> MTMATTAMNVSVPPPDEEEQLLAKFVFGDTTD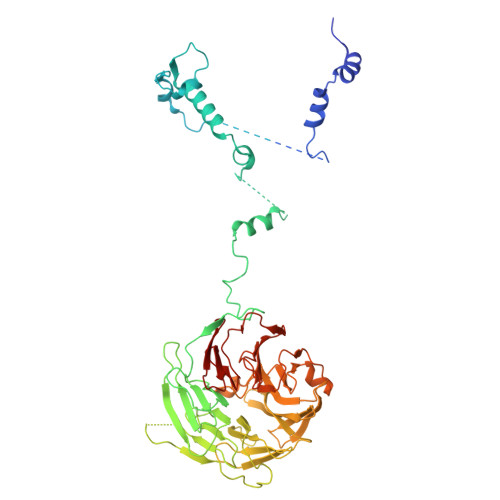LQENLAKFNADFIFNEQEMDVEDQEDEGSESDNSEEDEAQNGELDHVNNDQLFFVDDGGNEDSQDKNEDTMDVDDEDDSSSDDYSEDSEEAAWIDSDDEKIKVPILVTNKTKKLRTSYNESKINGVHYINRLRSQFEKIYPRPKWVDDESDSELDDEEDDEEEGSNNVINGDINALTKILSTTYNYKDTLSNSKLLPPKKLDIVRLKDANASHPSHSAIQSLSFHPSKPLLLTGGYDKTLRIYHIDGKTNHLVTSLHLVGSPIQTCTFYTSLSNQNQQNIFTAGRRRYMHSWDLSLENLTHSQTAKIEKFSRLYGHESTQRSFENFKVAHLQNSQTNSVHGIVLLQGNNGWINILHSTSGLWLMGCKIEGVITDFCIDYQPISRGKFRTILIAVNAYGEVWEFDLNKNGHVIRRWKDQGGVGITKIQVGGGTTTTCPALQISKIKQNRWLAVGSESGFVNLYDRNNAMTSSTPTPVAALDQLTTTISNLQFSPDGQILCMASRAVKDALRLVHLPSCSVFSNWPTSGTPLGKVTSVAFSPSGGLLAVGNEQGKVRLWKLNHY3-(2-methyl-1,3-thiazol-4-yl)aniline | C10 H10 N2 S | 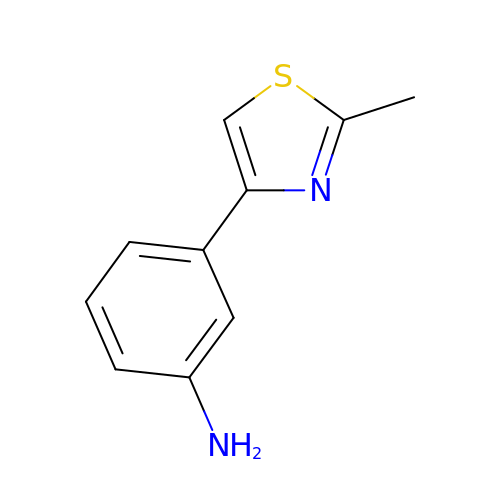CPHZPWZSSBCSAH-UHFFFAOYSA-N> ISEV;> QDSLPDTKASGPAHSKEVPALTAVETGATNPLAPSDTVQTRHVVQRRSRSESTIESFFARGACVAIIEVDNEQPTTRAQKLFAMWRITYKDTVQLRRKLEFFTYSRFDMEFTFVVTANFTNANNGHALNQVYQIMYIPPGAPTPKSWDDYTWQTSSNPSIFYTYGAAPARISVPYVGLANAYSHFYDGFAKVPLKTDANDQIGDSLYSAMTVDDFGVLAVRVVNDHNPTKVTSKVRIYMKPKHVRVWCPRPPRAVPYYGPGVDYRNNLDPLSEKGLTTY;> ACGYSDRVLQLTLGNSTITTQEAANSVVAYGRWPEFIRDDEANPVDQPTEPDVATCRFYTLDTVMWGKESKGWWWKLPDALRDMGLFGQNMYYHYLGRSGYTVHVQCNASKFHQGALGVFAIPEYCLAGDSDKQRYTSYANANPGERGGKFYSQFNKDNAVTSPKREFCPVDYLLGCGVLLGNAFVYPHQIINLRTNNSATIVLPYVNALAIDSMVKHNNWGIAILPLSPLDFAQDSSVEIPITVTIAPMCSEFNGLRNVTAPKFQ;> GLPVLNTPGSNQYLTSDNHQSPCAIPEFDVTPPIDIPGEVKNMMELAEIDTMIPLNLESTKRNTMDMYRVTLSDSADLSQPILCLSLSPAFDPRLSHTMLGEVLNYYTHWAGSLKFTFLFCGSMMATGKILVAYAPPGAQPPTSRKEAMLGTHVIWDLGLQSSCTMVVPWISNVTYRQTTQDSFTEGGYISMFYQTRIVVPLS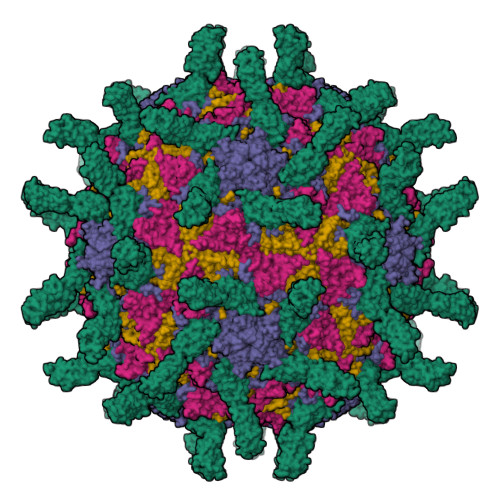TPKSMSMLGFVSACNDFSVRLLRDTTHISQSA;> GAQVSSQKVGAHENSNRAYGGSTINYTTINYYKDSASNAASKQDYSQDPSKFTEPLKDVLIKTAPALN;> VVQAPTQVPGFLGDSVTLPCYLQVPNMEVTHVSQLTWARHGESGSMAVFHQTQGPSYSESKRLEFVAARLGAELRDASLRMFGLRVEDEGSYTCLFVTFPQGSRSVDIWLRVLAKPQNTAEVQKVQLTGEPVPMARCVSTGGRPPAQITWHSDLGGMPQTSQVPGFLSGTVTVTSLWILVPSSQVDGKQVTCKVEHESFEKPQLLTVSLTVYY>[2x]MTKQEKTALNM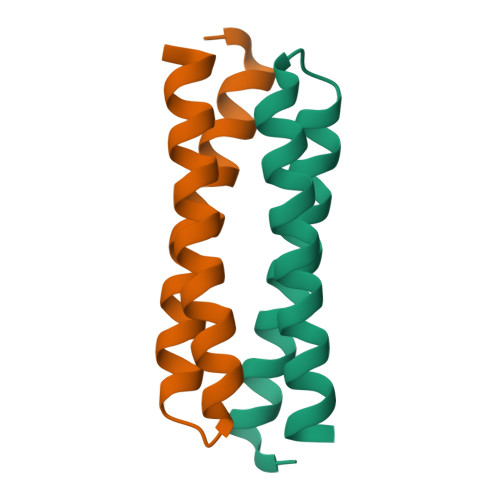ARFIRSQTLTLLEKLNELPGDEQADICESLHDHADELYRSCLARFGDDGENLEHHHHHH> MAVDSSNSATGPM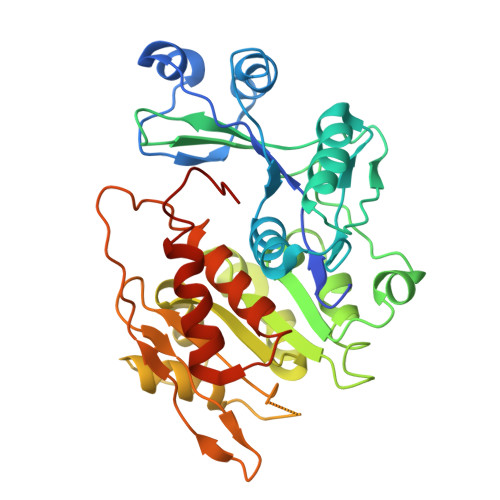RVFAIGNPILDLVAEVPSSFLDEFFLKRGDATLATPEQMRIYSTLDQFNPTSLPGGSALNSVRVVQKLLRKPGSAGYMGAIGDDPRGQVLKELCDKEGLATRFMVAPGQSTGTCAVLINEKERTLCTHLGACGSFRIPEDWTTFASGALIFYATAYTLTATPKNALEVAGYAHGIPNAIFTLNLSAPFCVELYKDAMQSLLLHTNILFGNEEEFAHLAKVHNLVAADKTALSTANKEHAVEVCTGALRLLTAGQNTGATKLVVMTRGHNPVIAAEQTADGTVVVHEVGVPVVAAEKIVDTNGAGDAFVGGFLYGLSQGKTVKQCIMCGNACAQDVIQHVGFSLSFTSLPC>[2x]SGLVKLGLWGGNEGTLQDIDGHPTRLTKIVIRSAHAIDALQFDYVEDGKTFAAGQWGGNGGKSDTIEFQPGEYLIAIKGTTGALGAVTNLV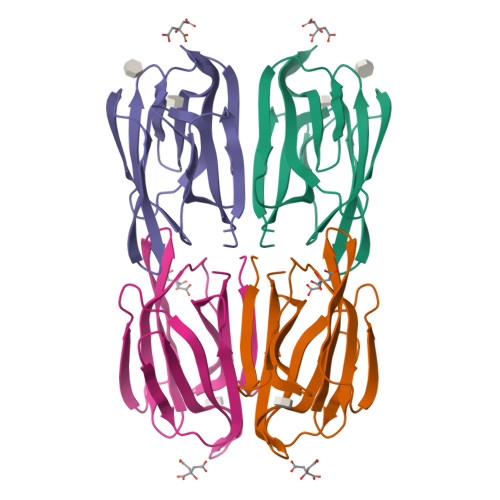RSLTFISNMRTYGPFGLEHGTPFSVPVASGRIVAFYGRFGSLVDAFGIYLMPY> MDRLTPLLSGWLDKLSPQGNYVFQRRFVQFNGRSLMYFGSDKDPFPKGVIPLTAIEMT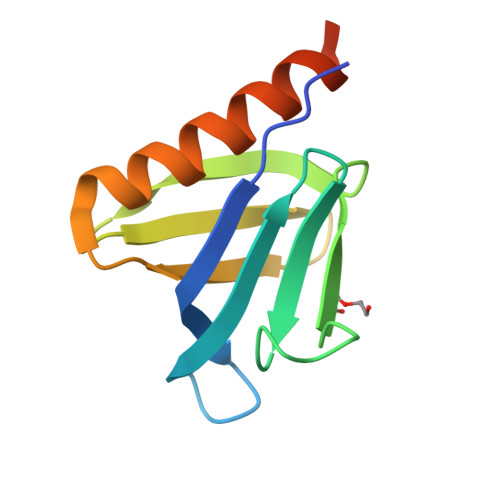RSSKDNKFQVITGQRVFVFRTESEAQRDMWCSTLQSCLKEQRLLGLEHHHHHH> MAALTPDLTTATPRLQYFHIAGPGTREYLSEDLQQFISATGSYFDLKNKFRQTVVAPTRNVTTEKAQRLQIRFYPIQTDDTSTGYRVRYNINVGDG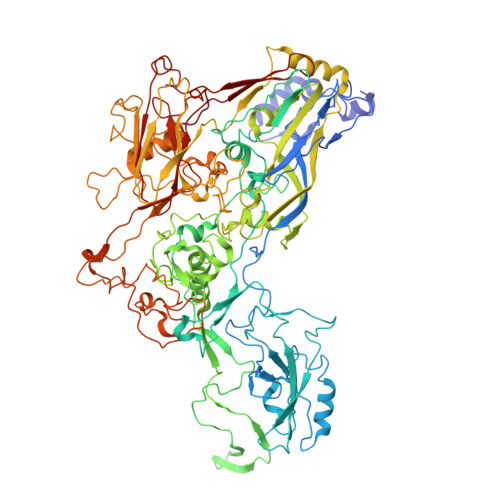WVLDMGSTYFDIKGILDRGPSFKPYCGTAYNPLAPKESMFNNWSETAPGQNVSASGQLSNVYTNTSTTKDTTAAQVTKISGVFPNPNQGPGINPLRQVENANTGVLGRFAKSQYNYAYGAYVKPVAADGSQSLTQTPYWIMNNAGTEYLGAVAVEDYTNSLSYPDTMIVPPPEDYDDYNIGTTRALRPNYIGFRDNFINLLYHDSGVCSGTLNSERSGMNVVVELPDRNTELSYQYMLADMMSRHHYFALWNQAVDQYDPEVRVFSNDGYEEGAPSYAFNPEAVGAGEGYGPDLSQIKLYTNNTAANDKNTAVTNATTNFYFGTVPSYEIDISATQRRNFIMANIAEYLPDRYKFSISGFDATSVAPTTYEYMNKRVPLTNVVDMFTNVGARWSIDQMDNVNPFNHHRNWGLKYRSQLLGNSRYVNFHIQVPQKFFAIKNLLLLSGSYTYEWVLRKDPNMILQSSLGNDLRADGASIIYNEVNLMANFMPMDHNTSNQLELMLRNATNDQTFVDYLGAKNALYSVPAGSTALTINIPARTWEGMRGWSFTRIKAAETPQLGAQYDVNFKYSGSIAYSDGGFYLSHTFRNMSILFDTSINWPGNDRLLTPNMFEIKRSVALDTEGFTMSQCDITKDWYLIQMATNYNFVYNGYRFWPDRQYFHYDFLRNFDPMTRQGPNFALPGLFDLVSYTPTTDNSGEQPSQEAVRNNSGFIAPRSWPVWSAHQGESWPANWPYPLCGQQAIQPGQVLSYKKFLCDNYLWTIPFSSDFMYMGELTDLGQNPMYTNNSHSMVINFELDPMDDPTYVYMLYGVFDTVRVNQPERNVLAMAYFRTPFATGNAV>[2x]MSKIEKLSILGVRSFGPHHPETIAFNTPLTLIVGYNGSGKTTVIECLKYATTGELPPNSTRNGAFIHDPDLVGEKEVRAQVKLSFRSTIGESYVVTRNIQLLVQRNNKRTQKTLEGSLLLRNNGERTVISTRVAELDKLVSEKLGVPPAILDAVIFCHQDDSLWPMSEPAALKKRFDEIFEAQKYTKVIENIRLLKKKKGDELKILKEREVQDKANKERAEKVDGGAGGAGGELDLKDAKAKYKETHI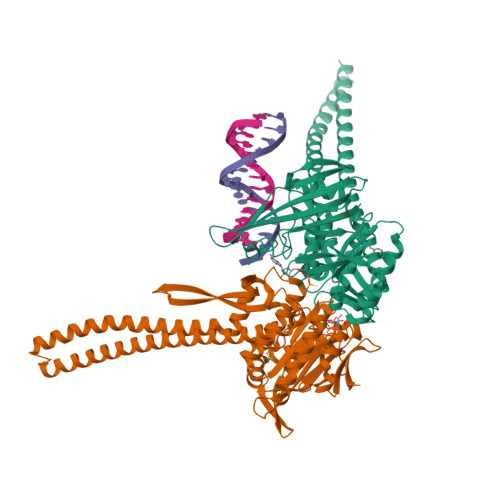KVETTKAAIEDLGRGMAAVDHAIMQYHSKMMEQINRTIAELWQSTYQGTDIDTIQIRSDVESTTSSDSGTRRNYNYRVSMVKGDTEMDMRGRCSAGQKVLASIIIRLALAESFCANCGLIALDQPTTNLDSDNIRSLAESLHGIIKARQAQGNLQLIVITHDEEFLKYMQCSDFCDDFYRVKRDEKQNSVIVRESITRITE> MGSDKIHHHHHHENLYFQGMEGYRLLYPMRTYLIVSGHGEETNVMAADWVTVVSFDPFIVGVAVAPKRTTHKLIKKYGEFVISVPSLDVLRDVWIAGTKKGPSKLKEMSVTLIPSKKVKVPSIEEALANIECRVIDARSYGDHTFFVGEVV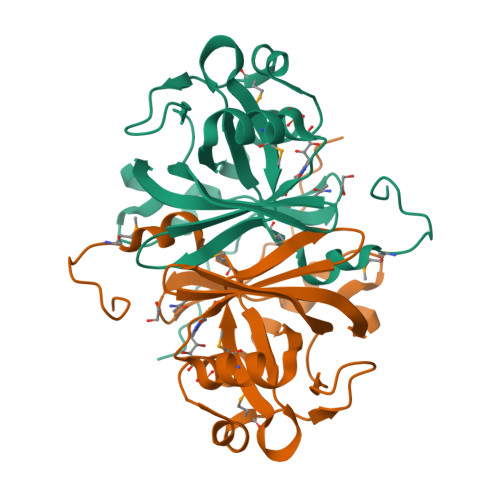GYTYKDYAFEKGKPNLKAKFLAHVSWSEFVTFSEKVHKAE> LSQAQKMQAIGQLAGGVAHDFNNLLTAIQLRLDELLHRHPVGDPSYEGLNEIRQTGVRAADLVRKLLAFSRKQTVQREVLDLGELISEFEVLLRRLLREDVKLITDYGRDLPQVRADKSQLETAVMNLAVNARDAVRAAKGGGVVRIRTARLTRDEAIQLGFPAAD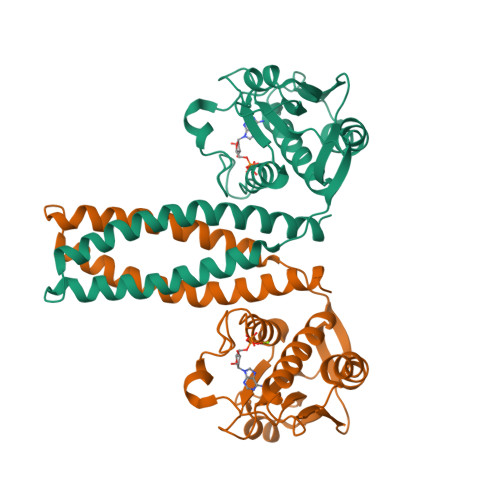GDTAFIEVSDDGPGIPPDVMGKIFDPFFTTKPVGEGTGLGLATVYGIVKQSDGWIHVHSRPNEGAAFRIFLPVYEA> SGIVQQQNNLLRAIEAQQHLLQLTVWGIKQLQARSGGRGGWMEWDREANNYTSLIHSLIEES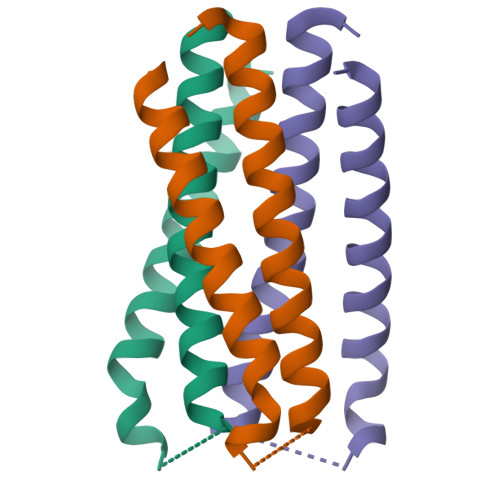QNQQEK> MSAKAISEQTGKELLYKFICTTSAIQNRFKYARVTPDTDWARLLQDHPWLLSQNLVVKPDQLIKRRGKLGLVGVNLTLDGVKSWLKPRLGQEATVGKATGFLKNFLIEPFVPHSQAEEFYVCIYATREGDYVLFHHEGGVDVGDVDAKAQKLLVGVDEKLNPEDIKKHLLVHAPEDKKEILASFISGLFNFYEDLYFTYLEINPLVVTKDGVYVLDLAAKVDATA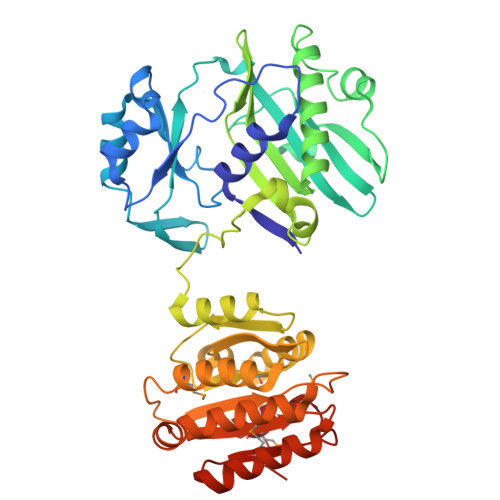DYICKVKWGDIEFPPPFGREAYPEEAYIADLDAKSGASLKLTLLNPKGRIWTMVAGGGASVVYSDTICDLGGVNELANYGEYSGAPSEQQTYDYAKTILSLMTREKHPDGKILIIGGSIANFTNVAATFKGIVRAIRDYQGPLKEHEVTIFVRRGGPNYQEGLRVMGEVGKTTGIPIHVFGTETHMTAIVGMALGHRPIP> GPGSASPDLLSEVSEMKQDLIKMTAI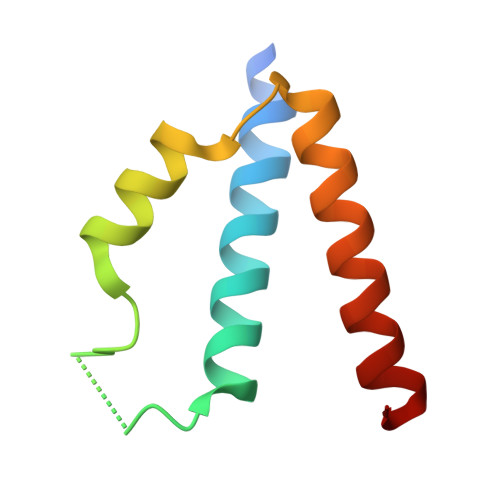LTTDVSDKAGSIKVKELVKAAEEEPGEPFEIVERVKEDLEKVNEILRSGT> FNKECLLRYKEAALDPNLNLYQRIAKIVSIDDDC;> HEVVKFMDVYQRSYCHPIETLVDIFQEYPDEIEYIFKPSCVPLMRCGGCCNDEGLECVPTEESNITMQIMRIKPHQGQHIGEMSFLQHN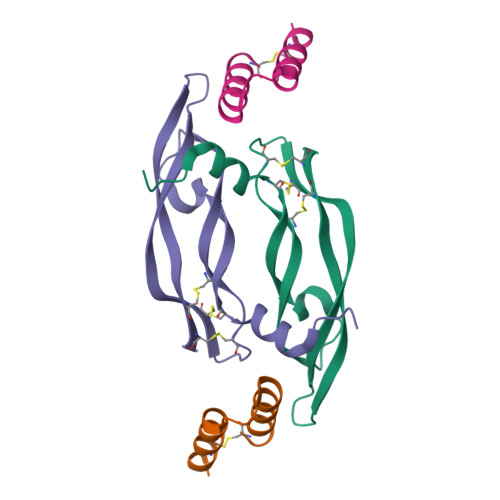KCECRPK>MRVLFIGDVMAEPGLRAVGLHLPDIRDRYDLVIANGENAARGKGLDRRSYRLLREAGVDLVSLGNHAWDHKEVYALLESEPVVRPLNYPPGTPGKGFWRLEVGGESLLFVQVMGRIFMDPLDDPFRALDRLLEEEKADYVLVEVHAEATSEKMALAHYLDGRASAVLGTHTHVPTLDATRLPKGTLYQTDVGMTGTYHSIIGGEVETFLARFLTGRPQPFRAAQGKARFHATELVFEGGRPVAISPYV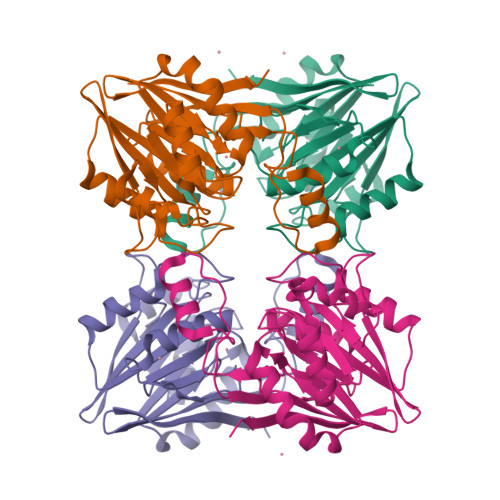WEEP[4x]> MVIQVTNKDEFESILSEADKLVVVDFTATWCGPCKMIAPKFEELSEEYPDNVVFLKVDVDEVE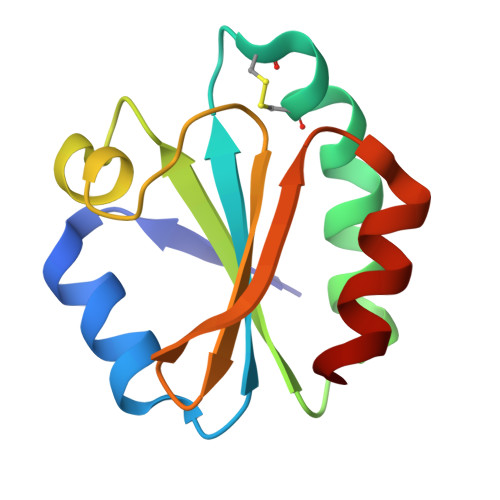DVAAEYGISAMPTFQFFKNGKKVDELTGANQEKLKAMIKKHAA PIEZO channels transmit mechanical force signals to cells, allowing them to make critical decisions during development and in pathophysiological conditions. Here, we report several near-atomic resolution cryo-EM structures of fast-inactivating wild-type human PIEZO1 (hPIEZO1) and its slow-inactivating channelopathy mutants with or without its auxiliary subunit MDFIC. Each hPIEZO1 subunit has a curved blade structure, and the three subunits form the trimeric PIEZO channel, exhibiting a bowl-like shape. MDFIC, a MyoD family inhibitor protein, has recently been identified as an auxiliary subunit of piezo channels capable of decelerating channel inactivation and attenuating channel mechanosensitivity.

The purified hPIEZO1 protein was subjected to the standard cryo-EM workflow, resulting in a cryo-EM density map at a total resolution of 3.3 Å from approximately 87K particles that allowed us to build a near-atomic model of hPIEZO1. The rest of the THUs, along with the pore module consisting of an anchor, an outer helix (OH), an IH, and a cap domain, are resolved. The hPIEZO1 density map, filtered with a low-pass filter, shows a disk approximately 30 nm wide with a horn-like density in the peripheral blade region, likely due to the PTMs such as glycosylation. Structural comparison of hPIEZO1 and curved mPIEZO1 shows that hPIEZO1 presents a more flattened structure from the side view. The blades of hPIEZO1 are about 5 Å down toward the cytoplasmic side than those of mPIEZO1. Therefore, hPIEZO1 appears more extended than the curved mPIEZO1. The pore radius of hPIEZO1 is between that of the curved and flattened mPIEZO1. Therefore, the curved hPIEZO1 may still represent a nonconducting state, and the differences in curvature and pore radius may be implicated in channel gating properties of hPIEZO1 and mPIEZO1. We also carefully checked the corresponding pore lipid configuration in the 3.3 Å resolution map of hPIEZO1 and the 3.8 Å resolution map of hPIEZO1-A1988V without the multi-lipidated MDFIC auxiliary subunit and found that in wild-type hPIEZO1, similar pore lipids also insert into the hydrophobic pore interacting with R2456. Our high-resolution structures support a model in which the pore lipids directly seal the central hydrophobic pore and involve fast inactivation of hPIEZO1.

>[3x]MEPHVLGAVLYWLLLPCALLAACLLRFSGLSLVYLLFLLLLPWFPGPTRCGLQGHTGRLLRALLGLSLLFLVAHLALQICLHIVPRLDQLLGPSCSRWETLSRHIGVTRLDLKDIPNAIRLVAPDLGILVVSSVCLGICGRLARNTRQSPHPRELDDDERDVDASPTAGLQEAATLAPTRRSRLAARFRVTAHWLLVAAGRVLAVTLLALAGIAHPSALSSVYLLLFLALCTWWACHFPISTRGFSRLCVAVGCFGAGHLICLYCYQMPLAQALLPPAGIWARVLGLKDFVGPTNCSSPHALVLNTGLDWPVYASPGVLLLLCYATASLRKLRAYRPSGQRKEAAKGYEARELELAELDQWPQERESDQHVVPTAPDTEADNCIVHELTGQSSVLRRPVRPKRAEPREASPLHSLGHLIMDQSYVCALIAMMVWSITYHSWLTFVLLLWACLIWTVRSRHQLAMLCSPCILLYGMTLCCLRYVWAMDLRPELPTTLGPVSLRQLGLEHTRYPCLDLGAMLLYTLTFWLLLRQFVKEKLLKWAESPAALTEVTVADTEPTRTQTLLQSLGELVKGVYAKYWIYVCAGMFIVVSFAGRLVVYKIVYMFLFLLCLTLFQVYYSLWRKLLKAFWWLVVAYTMLVLIAVYTFQFQDFPAYWRNLTGFTDEQLGDLGLEQFSVSELFSSILVPGFFLLACILQLHYFHRPFMQLTDMEHVSLPGTRLPRWAHRQDAVSGTPLLREEQQEHQQQQQEEEEEEEDSRDEGLGVATPHQATQVPEGAAKWGLVAERLLELAAGFSDVLSRVQVFLRRLLELHVFKLVALYTVWVALKEVSVMNLLLVVLWAFALPYPRFRPMASCLSTVWTCVIIVCKMLYQLKVVNPQEYSSNCTEPFPNSTNLLPTEISQSLLYRGPVDPANWFGVRKGFPNLGYIQNHLQVLLLLVFEAIVYRRQEHYRRQHQLAPLPAQAVFASGTRQQLDQDLLGCLKYFINFFFYKFGLEICFLMAVNVIGQRMNFLVTLHGCWLVAILTRRHRQAIARLWPNYCLFLALFLLYQYLLCLGMPPALCIDYPWRWSRAVPMNSALIKWLYLPDFFRAPNSTNLISDFLLLLCASQQWQVFSAERTEEWQRMAGVNTDRLEPLRGEPNPVPNFIHCRSYLDMLKVAVFRYLFWLVLVVVFVTGATRISIFGLGYLLACFYLLLFGTALLQRDTRARLVLWDCLILYNVTVIISKNMLSLLACVFVEQMQTGFCWVIQLFSLVCTVKGYYDPKEMMDRDQDCLLPVEEAGIIWDSVCFFFLLLQRRVFLSHYYLHVRADLQATALLASRGFALYNAANLKSIDFHRRIEEKSLAQLKRQMERIRAKQEKHRQGRVDRSRPQDTLGPKDPGLEPGPDSPGGSSPPRRQWWRPWLDHATVIHSGDYFLFESDSEEEEEAVPEDPRPSAQSAFQLAYQAWVTNAQAVLRRRQQEQEQARQEQAGQLPTGGGPSQEVEPAEGPEEAAAGRSHVVQRVLSTAQFLWMLGQALVDELTRWLQEFTRHHGTMSDVLRAERYLLTQELLQGGEVHRGVLDQLYTSQAEATLPGPTEAPNAPSTVSSGLGAEEPLSSMTDDMGSPLSTGYHTRSGSEEAVTDPGEREAGASLYQGLMRTASELLLDRRLRIPELEEAELFAEGQGRALRLLRAVYQCVAAHSELLCYFIIILNHMVTASAGSLVLPVLVFLWAMLSIPRPSKRFWMTAIVFTEIAVVVKYLFQFGFFPWNSHVVLRRYENKPYFPPRILGLEKTDGYIKYDLVQLMALFFHRSQLLCYGLWDHEEDSPSKEHDKSGEEEQGAEEGPGVPAATTEDHIQVEARVGPTDGTPEPQVELRPRDTRRISLRFRRRKKEGPARKGAAAIEAEDREEEEGEEEKEAPTGREKRPSRSGGRVRAAGRRLQGFCLSLAQGTYRPLRRFFHDILHTKYRAATDVYALMFLADVVDFIIIIFGFWAFGKHSAATDITSSLSDDQVPEAFLVMLLIQFSTMVVDRALYLRKTVLGKLAFQVALVLAIHLWMFFILPAVTERMFNQNVVAQLWYFVKCIYFALSAYQIRCGYPTRILGNFLTKKYNHLNLFLFQGFRLVPFLVELRAVMDWVWTDTTLSLSSWMCVEDIYANIFIIKCSRETEKKYPQPKGQKKKKIVKYGMGGLIILFLIAIIWFPLLFMSLVRSVVGVVNQPIDVTVTLKLGGYEPLFTMSAQQPSIIPFTAQAYEELSRQFDPQPLAMQFISQYSPEDIVTAQIEGSSGALWRISPPSRAQMKRELYNGTADITLRFTWNFQRDLAKGGTVEYANEKHMLALAPNSTARRQLASLLEGTSDQSVVIPNLFPKYIRAPNGPEANPVKQLQPNEEADYLGVRIQLRREQGAGATGFLEWWVIELQECRTDCNLLPMVIFSDKVSPPSLGFLAGYGIMGLYVSIVLVIGKFVRGFFSEISHSIMFEELPCVDRILKLCQDIFLVRETRELELEEELYAKLIFLYRSPETMIKWTREKE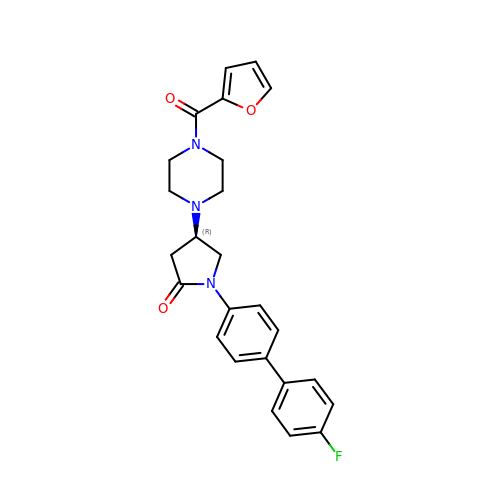(4~{R})-1-[4-(4-fluorophenyl)phenyl]-4-[4-(furan-2-ylcarbonyl)piperazin-1-yl]pyrrolidin-2-one | C25 H24 F N3 O3 | HVVLTSHAUJYILM-JOCHJYFZSA-N>SHMDPVSVWGNTPLATVDPEIHDLIEKEKRRQCRGIELIASENFTSFAVIEALGSALTNKYSEGMPGNRYYGGNEYIDQIENLCRSRALQAFHLDAQSWGVNVQPYSGSPANFAAYTAVLNPHDRIMGLDLPSGGHLTHGYYTSGGKKISATSIYFESLPYKVNSTTGYIDYDRLEEKALDFRPKLIICGGSAYPRDWDYKRFREVADKCGALLLCDMAHTSGLVAAQEVNSPFEYCDIVTTTTHKSLRGPRAGMIFYRKGPKPPKKG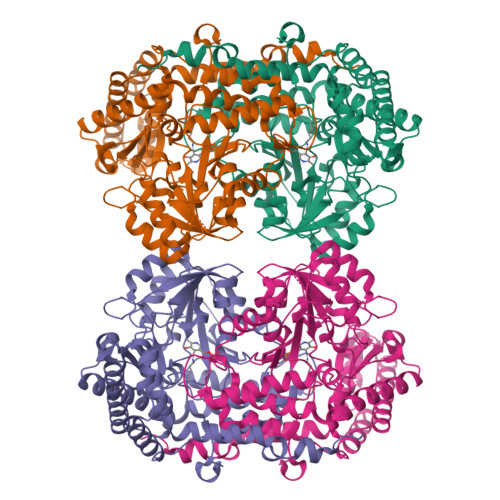QPENAVYDFEDKINFAVFPSLQGGPHNHQIGALAVALKQAASPGFKAYAKQVKANAVALGKYLMGKGYSLVTGGTENHLVLWDLRPLGLTGNKVEKLCDLCNITVNKNAVFGDSSALAPGGVRIGAPAMTSRGLVEKDFEQIGEFLHRAVTLTLEIQKEHGKLLKDFNKGLVNNKAIEDLKADVEKFSALFDMPGFLVSEMKYKD[2x]> MSGLAK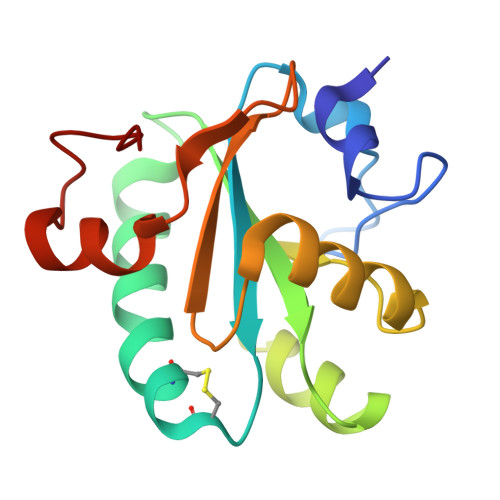YLPGATNLLSKSGEVSLGSLVGKTVFLYFSASWCPPCRGFTPVLAEFYEKHHVAKNFEVVLISWDENESDFHDYYGKMPWLALPFDQRSTVSELGKTFGVESIPTLITINADTGAIIGTQARTRVIEDPDGANFPWPN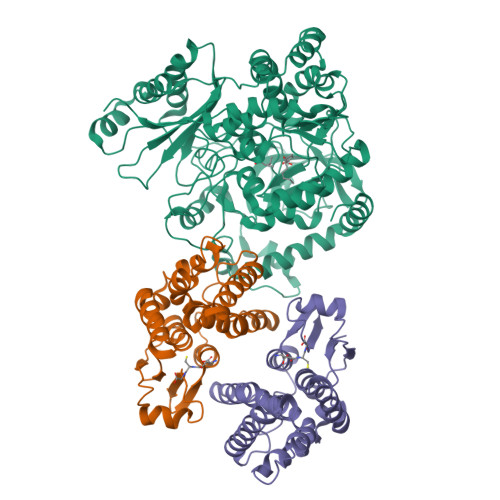>MLEKVETFDMNRVIDEFDEMTRNAHQVQKQTLKEILLKNQSAIYLQNCGLNGNATDPEEAFKSMVPLVTDVELEPYIKRMVDGDTSPILTGHPVPAISLSSGTSQGRPKFIPFTDELMENTLQLFRTAFAFRNRDFPIDDNGKALQFIFSSKQYISTGGVPVGTATTNVYRNPNFKAGMKSITSPSCSPDEVIFSPDVHQALYCHLLSGILFRDQVQYVFAVFAHGLVHAFRTFEQVWEEIVTDIKDGVLSNRITVPSVRTAMSKLLTPNPELAETIRTKCMSLSNWYGLIPALFPNAKYVYGIMTGSMEPYVPKLRHYAGDLPLVSHDYGSSEGWIAANVTPRLSPEEATFAVIPNLGYFEFLPVSETGEGEEKPVGLTQVKIGEEYEVVITNYAGLYRYRLGDVVKVIGFYNNTPQLKFICRRNLILSINIDKNTERDLQLSVESAAKRLSEEKIEVIDFSSYIDVSTDPGHYAIFWEISGETNEDVLQDCCNCLDRAFIDAGYVSSRKCKTIGALELRVVAKGTFRKIQEHFLGLGSSAGQFKMPRCVKPSNAKVLQILCENVVSSYFSTAF[2x];>[4x]HHHHHHMANLPILLDYWPSMFGMRARVALREKGVEFEYREEDFSNKSPLLLQSNPIHKKIPVLVHNGKPVCESLNVVQYVDEAWPEKNPFFPSDPYGRAQARFWADFVDKKFTDAQFKVWGKKGEEQEAGKKEFIEAVKILESELGDKPYFGGDSFGYVDISLITFSSWFQAYEKFGNFSIESESPKLIAWAKRCMEKESVSKSLPDSEKIVAYAAEYRKNNL> MHPETLVKVKDAEDQLGARVGYIELDLNSGKILESFRPEERFPMMSTFKVLLCGAVLSRIDAGQEQLGRRIHYSQNDLVEYSPVTEKHLTDGMTVRELCSAAITMSDNTAANLLLTTIGGPKELTAFLHNMGDHVTRLDRWEPELNEAIPNDERDTTMPAAMATTLRKLLTGELLTLASRQQLIDWMEADKVAGPLLRSAL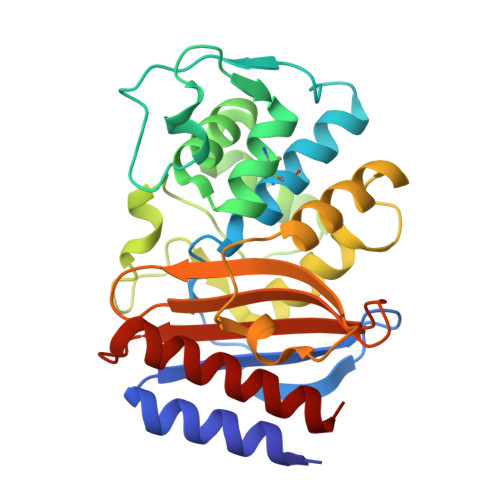PAGWFIADKSGAGERGSRGIIAALGPDGKPSRIVVIYTTGSQATMDERNRQIAEIGASLIKHW>[4x]DSISLSLINEGPSYASKVSVGSNKQQQTVIIDTGSSDFWVVDSNAQCGKGVDCKSSGTFTPS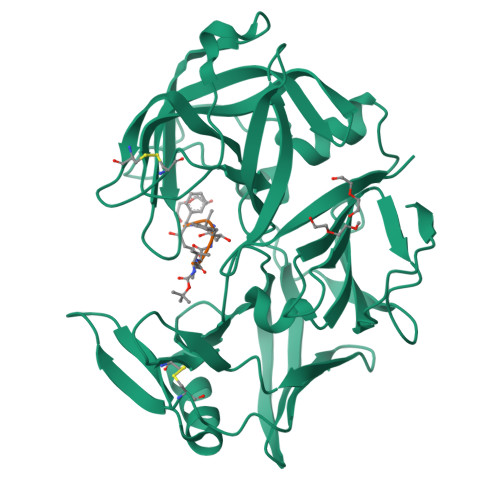SSSSYKNLGAAFTIRYGDGSTSQGTWGKDTVTINGVSITGQQIADVTQTSVDQGILGIGYTSNEAVYDTSGRQTTPNYDNVPVTLKKQGKIRTNAYSLYLNSPSAETGTIIFGGVDNAKYSGKLVAEQVTSSQALTISLASVNLKGSSFSFGDGALLDSGTTLTYFPSDFAAQLADKAGARLVQVARDQYLYFIDCNTDTSGTTVFNFGNGAKITVPNTEYVYQNGDGTCLWGIQPSDDTILGDNFLRHAYLLYNLDANTISIAQVKYTTDSSISAV;>XVVFAFA[4x]>[2x]MNLPTAQEVQGLMARYIELVDVGDIEAIVQMYADDATVEDPFGQPPIHGREQIAAFYRQGLGGGKVRACLTGPVRASHNGCGAMPFRVEMVWNG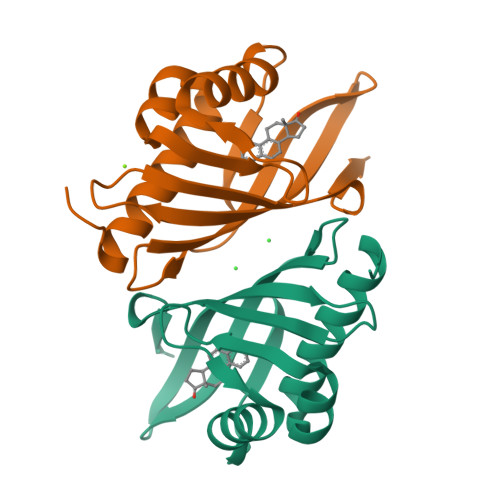QPCALDVIDVMRFDEHGRIQTMQAYWSEVNLSVREPQ>GKSVVTLKTTDGWIPVPFSKVMYLEAKDKKTYVNAEELTGTHKYSLQEFEYLLPKDSFIRCHRSFIVNVNHIK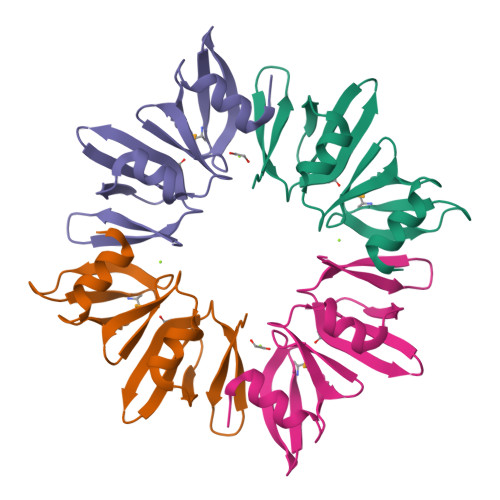AIYPDTHSTFLLSMDNGERVPVSQSYASYFRKLLGFGS[2x]> MNNSSELIAVINGFRNSGRFCDISIVINDERINAHKLILSGASEYFSILFSNNFIDSNEYEVNLSHLDYQSVNDLIDYIYGIPLSLTNDNVKYILSTADFLQIGSAITECENYILKNLCSKNCIDFYIYADKYNNKKIESASFNTILQNILRLINDENFKYLTEESMIKILSDDMLNIKNEDFAPLILIKWLESTQQSCTVELLRCLRISLLSPQVIKSLYSHQLVSSIYECITFLNNIAFLDESFPRYHGSKHHHHHH;> MTMDEKYVNSIWDLLKNAIQEIQRKNNSGLSFEELYRNAYTMVLHKHGEKLYTGLREVVTEHLINKVREDVLNSLNNNFLQTLNQAWNDHQTAMVMIRDILMYMDRVYVQQNNVENVYNLGLIIFRDQVVRYGCIRDHLRQTLLDMIARERKGEVVDRGAIRNACQMLMILGLEGRSVYEEDFEAPFLEMSAEFFQMESQKFLAENSASVYIKKVEARINEEIERVMHCLDKSTEEPIVKVVERELISKHMKTIVEMENSGLVHMLKNGKTEDLGCMYKLFSRVPNGLKTMCECMSSYLREQGKALVSEEGEGKNPVDYRQGLDDLKSRFDRFLLESFNNDRLFKQTIAGDFEYFLNLNSRSPEYLAENLYFQSHHHHHHDYKDDDDK

A55 is an intracellular protein encoded by the A55R gene of VACV. It belongs to the BTB (Bric-a-brac, Tramtrack, and Broad complex)-Kelch protein family, which are substrate adaptor proteins specific for the cullin-3 (Cul3)-RING (Really Interesting New Gene)–based E3 ubiquitin ligase (C3RL) complex. The N-terminal region of these proteins contains a BTB domain that mediates dimerization and binding to Cul3, a three-box helical bundle region, and a BACK (for BTB and C-terminal Kelch) domain that is likely responsible for correctly orienting the C terminus. In this study, we showed that A55 binds directly to Cul3 and solved the crystal structure of a complex between Cul3–NTD and the BTB-BACK (BB) domain of A55.

To promote crystallization, A55BB was subjected to surface entropy reduction by reductive methylation before being purified in complex with Cul3NΔ22. To understand the molecular basis of this tight interaction, the crystal structure of the A55BB/Cul3NΔ22 complex was determined using anisotropic diffraction data extending to 2.3 Å (with an observation/parameter ratio equivalent to that of an isotropic 2.8 Å resolution structure). The structure of the A55BB(M)/Cul3NΔ22 complex contains one copy of each molecule in the crystallographic asymmetric unit. Consistent with the SEC-MALS analysis, a heterotetramer of A55BB(M)/Cul3NΔ22 can be observed by applying crystallographic 2-fold symmetry. A55BB dimerization is mediated by the BTB domain, where the N-terminal helix (α1) forms a domain-swapped interaction with the symmetry-related molecule. A55BB consists of a globular BTB domain (residues 1–118; helices α1–α6 and strands β2–β4) followed by a helix–turn–helix three-box region (residues 119–149; helices α7–α8) and an all-helical BACK domain (residues 150–196, helices α9–α12). The A55-binding interface of Cul3–NTD is formed primarily of residues in helices α2 and α5, with extra contacts from the α1–α2 loop and from the C terminus of α3. Residues at the Cul3-binding interface of A55BB are primarily found in the BTB domain with additional contacts in the three-box region; the BACK domain does not contribute to the interaction. However, compared with other BTB/Cul3–NTD structures, the A55BB/Cul3 interface has more hydrogen bonds and a reduced contribution from hydrophobic interactions. Residue Ile-48 of A55 is adjacent to the φ residue Phe-54 and, like Phe-54, the side chain of Ile-48 extends into a hydrophobic cleft on the Cul3 surface.>[3x]VDFHGYARSGIGWTGSGGEQQCFQTTGAQSKYRLG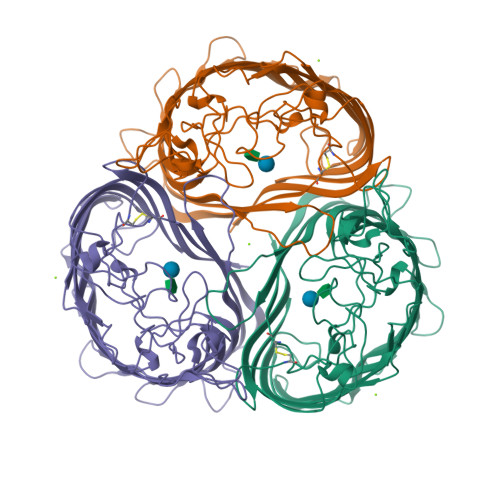NECETYAELKLGQEVWKEGDKSFYFDTNVAYSVAQQNDWEATDPAFREANVQGKNLIEWLPGSTIWAGKRFYQRHDVHMIDFYYWDISGPGAGLENIDVGFGKLSLAATRSSEAGGSSSFASNNIYDYTNETANDVFDVRLAQMEINPGGTLELGVDYGRANLRDNYRLVDGASKDGWLFTAEHTQSVLKGFNKFVVQYATDSMTSQGKGLSQGSGVAFDNEKFAYNINNNGHMLRILDHGAISMGDNWDMMYVGMYQDINWDNDNGTKWWTVGIRPMYKWTPIMSTVMEIGYDNVESQRTGDKNNQYKITLAQQWQAGDSIWSRPAIRVFATYAKWDEKWGYDYTGNADNNANFGKAVPADFNGGSFGRGDSDEWTFGAQMEIWW>PSVYDAAAQLTADVKKDLRDSWKVIGSDKKGNGVALMTTLFADNQETIGYFKRLGDVSQGMANDKLRGHSIILMYALQNFIDQLDNPDDLVCVVEKFAVNHITRKISAAEFGKINGPIKKVLASKNFGDKY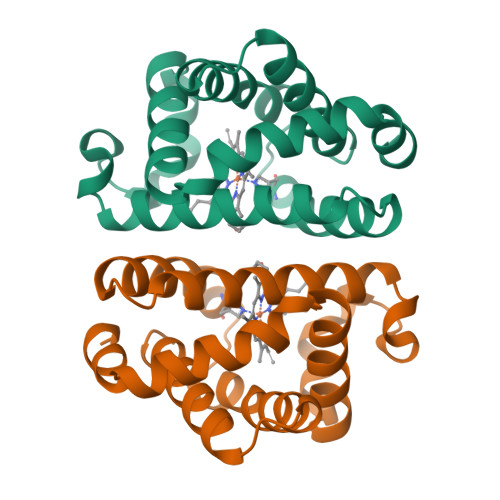ANAWAKLVAVVQAAL[2x]> LGEPRYA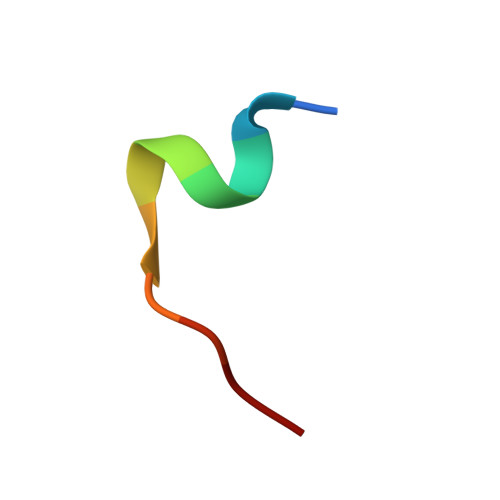FNFN2,2,3,3,4,4,4-heptafluorobutan-1-ol | C4 H3 F7 O 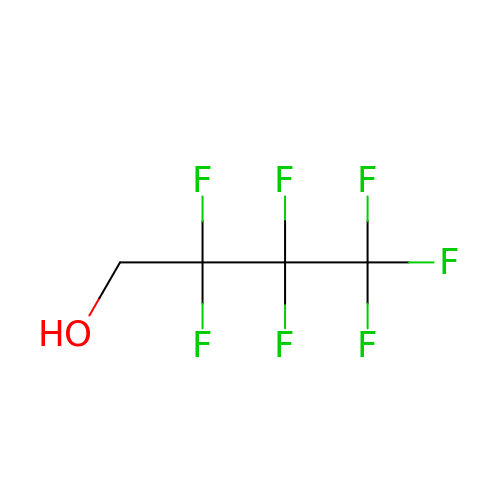| WXJFKAZDSQLPBX-UHFFFAOYSA-N>[4x]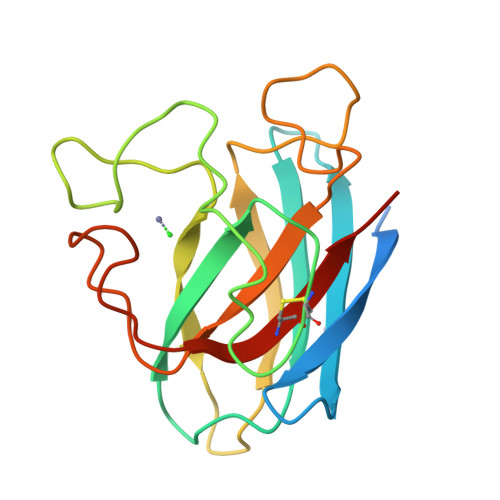KPPDPPNRVPEKKVVETSAFGHHVQLVNREGKAVGFIEIKESDDEGLDIHISANSLRPGASLGFHIYEKGSCVRPDFESAGGPFNPLNKEHGFNNPMGHHAGDLPNLEVGADGKVDVIMNAPDTSLKKGSKLNILDEDGSAFIIHEQADDYLTNPSGNSGARIVCGALLGNNEKQ> MRGSHHHHHHGSSYQIAVLAGDGIGPEVMAEARKVLKAVEARFGLNIEYTEYDVGGIAIDNHGCPLPEATLKGCEAADAILFGSVGGPKWEKLPPNEQPERGALLPLRGHFELFCNLRPAKLHDGLEHMSPLRSDISARGFDVLCVRELTGGIYFGKPKGRQGEGESEEAFDTMRYSRREISRIARIAFEAARGRRKKVTSVDKANVLACSVLWRQVVEEVAVDFPDVELEHIYIDNATMQLLRRPDEFDVMLCSNLFGDILSDEIAMLTGSMGLLSSASMNSTGFGLFEPAGGSAPDIAGKGIANPIAQILSAALMLRHSLKQEEAASAIERAVTKALNSGYLTGELLSSDQRHKAKTTVQMGDFIADAVKAGV

In this study, structures of 3-isopropylmalate dehydrogenase (IPMDH) from Shewanella oneidensis MR-1 were determined at about 2 Å resolution under pressures ranging from 0.1 to 650 MPa using a diamond anvil cell (DAC). IPMDH catalyzes the reduction of 3-isopropylmalate (IPM) to 2-­isopropyl-3-oxosuccinate in the presence of divalent metal cations such as magnesium or manganese ion and nicotin­amide adenine dinucleotide. In this study, the SoIPMDH dimer was crystallized in complex with its substrate, the IPM molecule. As a consequence, the SoIPMDH dimer adopts a closed conformation through binding IPM.

2 Å resolution crystal structures of the SoIPMDH–IPM complex were determined at room temperature at pressures of 0.1, 160, 340, 410, 580 and 650 MPa. In the structures at 0.1–650 MPa, with the exception of flexible loops on the surface of SoIPMDH and residues that adopt indistinct multiple conformations, no characteristic structural changes were observed. The volume of this cavity shows an initial decrease in volume, with values of 55.6 and 50.4 Å3 at pressures of 0.1 and 160 MPa, respectively, followed by a constant volume increase with values of 54.2, 57.6, 64.7 and 65.5 Å3 at 340, 410, 580 and 650 MPa, respectively. No electron density could be observed in the cavity at 0.1 MPa, while at 580 MPa two peaks were clearly visible. In the case of SoIPMDH, the volume of the cavity at the dimer interface is only 56 Å3 at 0.1 MPa and reduces slightly to 50 Å3 at 160 MPa. In the structures at pressures ranging from 0.1 to 410 MPa, the solvent-excluded surface at the bottom of the groove is nonpolar since it is mostly composed of the Pro108 and Leu305 side chains.> MNKRGLYSKLGISVVGISLLMGVPTLIHANELNYGQLSISPIFQGGSYQLNNKSIDISSLLLDKLSGESQTVVMKFKADKPNSLQALFGLSNSKAGFKNNYFSIFMRDSGEIGVEIRDAQKGINYLFSRPASLWGKHKGQAVENTLVFVSDSKDKTYTMYVNGIEVFSETVDTFLPISNINGIDKATLGAVNREGKEH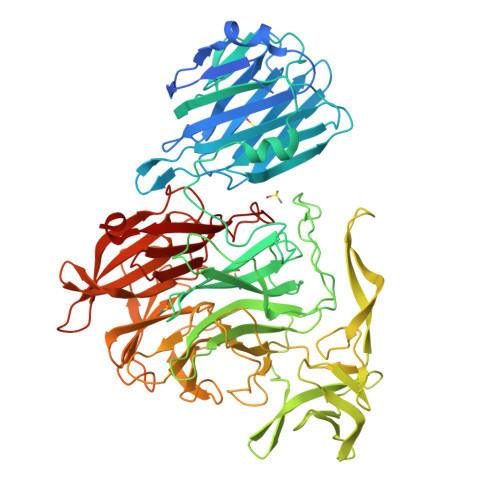YLAKGSIDEISLFNKAISDQEVSTIPLSNPFQLIFQSGDSTQANYFRIPTLYTLSSGRVLSSIDARYGGTHDSKSKINIATSYSDDNGKTWSEPIFAMKFNDYEEQLVYWPRDNKLKNSQISGSASFIDSSIVEDKKSGKTILLADVMPAGIGNNNANKADSGFKEINGHYYLKLKKNGDNDFRYTVRENGVVYNETTNKPTNYTINDKYEVLEGGKSLTVEQYSVDFDSGSLRERHNGKQVPMNVFYKDSLFKVTPTNYIAMTTSQNRGESWEQFKLLPPFLGEKHNGTYLCPGQGLALKSSNRLIFATYTSGELTYLISDDSGQTWKKSSASIPFKNATAEAQMVELRDGVIRTFFRTTTGKIAYMTSRDSGETWSKVSYIDGIQQTSYGTQVSAIKYSQLIDGKEAVILSTPNSRSGRKGGQLVVGLVNKEDDSIDWKYHYDIDLPSYGYAYSAITELPNHHIGVLFEKYDSWSRNELHLSNVVQYIDLEINDLTK> MRRCSFASTCRYRSADDVPLGLGSAYVWTCRNITSRGQFNPIHNFSYAMERGVRARDVKAFEKLITNPGPLRVAYTPDYLDWLHRCYKAKGTYMDARAVAEKKFNGNIVSSELSAAVNRREG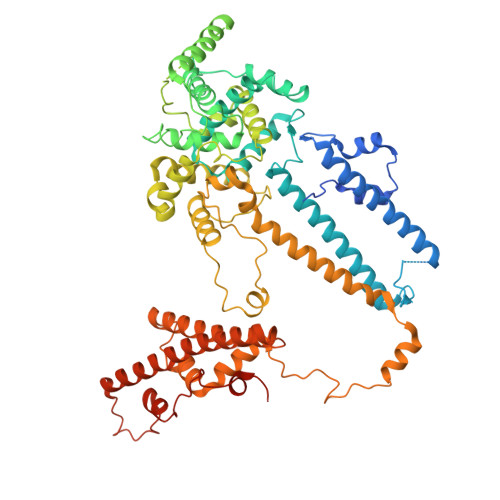KRGDTRGDTVDNDHHNLPGAPPPGMFLRPAHSFRRLAGELKRRRAQSILDEVARAQGMLDLFERQPHFPAIHIDRCSRFHLVELFKEMVLERSLDSNMIWEKALLYRAILSERKPSYPTSFHYIFTAVEDTVFAPTISTPMEMAGSGGEGHDRSSHPLAAKCPTLEAYYYYVYLVKKYYIDNAVEAHVVLRCHREPNAADLLFSNPPPKDDTEIMKAVELLRNADIQRGVAAAAAVSDPTLPPGGEGSVIGNSDNKKNSEKTSEGSRGRPARPPVLPGAYPPIDMLWRCEENLPLLKVLLFGEFNLIVSENPFVKFPSAHGFLTRPYSTDSSRTLADGMSLANVMAEKRGHLLPSLPRNTATSIDARAQDIRRLQQKHHRDDIVSFQKLLRSTHAEDSPSAFSSYSDWSYFNPRAVRAEERDRLTRKAVEALKLYDSATNDIYRHSFEDVQACHTQRVTERDRTMPPYLPTLPHFVAIIKKDPHISFLLHIGLPDRNSSEEGSAKHKELEKRIYYLARALYHTALEYHNETVRRVNRQKVNVAASLLDNFVEQEWTTILRDKHDVTDVTKTLNDTQNDKKQLARRLGRYMLFANRSLDDTGFPTDARADDYTRWMAPPSVGKVSL>[2x]GDNDPLVVNTDKGRIRGITVDAPSGKKVDVWLGIPYAQPPVGPLRFRHPRPAEKWTGVLNTTTPPNSCVQIVDTVFGDFPGATMWNPNTPLSEDCLYINVVAPRPRPKNAAVMLWIFGGSFYSGTATLDVYDHRALASEENVIVVSLQYRVASLGFLFLGTPEAPGNAGLFDQNLALRWVRDNIHRFGGDPSRVTLFGESAGAVSVSLHLLSALSRDLFQRAILQSGSPTAPWALVSREEATLRALRLAEAVGCPHEPSKLSDAVECLRGKDPHVLVNNEWGTLGICEFPFVPVVDGAFLDETPQ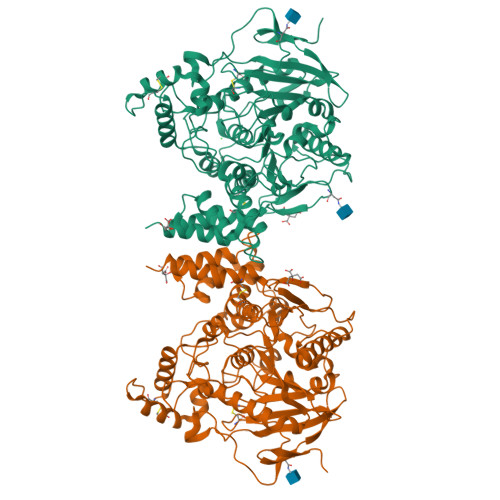RSLASGRFKKTEILTGSNTEEGYYFIIYYLTELLRKEEGVTVTREEFLQAVRELNPYVNGAARQAIVFEYTDWTEPDNPNSNRDALDKMVGDYHFTCNVNEFAQRYAEEGNNVYMYLYTHRSKGNPWPRWTGVMHGDEINYVFGEPLNPTLGYTEDEKDFSRKIMRYWSNFAKTGNPNPNTASSEFPEWPKHTAHGRHYLELGLNTSFVGRGPRLRQCAFWKKYLPQLVAATSNLPG>MAKKTSSTVLPFEAMPQHPGNRWLRLLQIWREQGYEHLHLEMHQTFQELGPIFRYNLGGPRMVCVMLPEDVEKLQQVDSLHPCRMILEPWVAYRQHRGHKCGVFLLNGPEWRFNRLRLNPDVLSPKAVQRFLPMVDAVARDFSQALKKKVLQNARGSLTLDVQPSIFHYTIEASNLALFGERLGLVGHSPSSASLNFLHALEVMFKSTVQLMFMPRSLSRWISPKVWKEHFEAWDCIFQYGDNCIQKIYQELAFNRPQHYTGIVAELLLKAELSLEAIKANSMELTAGSVDTTAFPLLMTLFELARNPDVQQILRQESLAAAASISEHPQKATTELPLLRAALKETLRLYPVGLFLERVVSSDLVLQNYHIPAGTLVQVFLYSLGRNAALFPRPE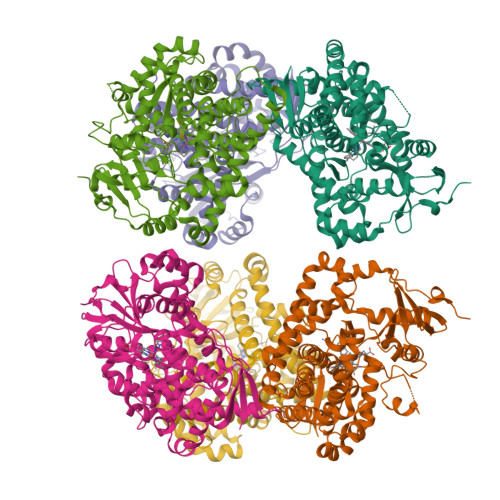RYNPQRWLDIRGSGRNFHHVPFGFGMRQCLGRRLAEAEMLLLLHHVLKHFLVETLTQEDIKMVYSFILRPGTSPLLTFRAINHHHHHH[12x]>[6x]MSLPTEMHHNLGAEKRSAVATTIDSFKERSQKVRALSDPNVRFVPFFGSSEWLRFDGAHPAVLAEKYNRSYRPYLLGQGGAASL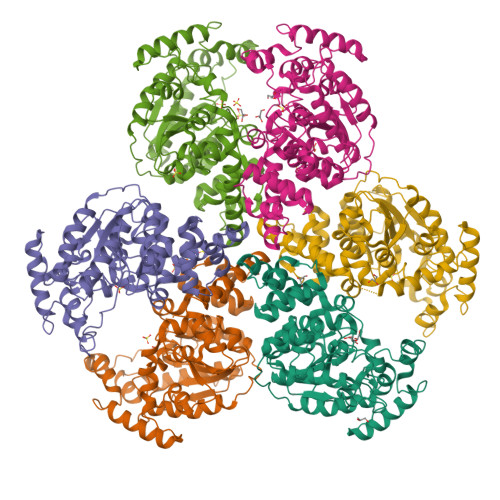NQYFGMQQMLPQLENKQVVYVISPQWFSKNGYDPAAFQQYFNGDQLTSFLKHQSGDQASQYAATRLLQQFPNVAMKDLVQKLASKEELSTADNEMIELLARFNERQASFFGQFSVRGYVNYDKHVAKYLKILPDQFSYQAIEDVVKADAEKNTSNNEMGMENYFYNEQIKKDLKKLKDSQKSFTYLKSPEYNDLQLVLTQFSKSKVNPIFIIPPVNKKWMDYAGLREDMYQQTVQKIRYQLESQGFTNIADFSKDGGEPFFMKDTIHLGWLGWLAFDKAVDPFLSNPTPAPTYHLNERFFSKDWATYDGDVKEFQEGHHHHHH>MHHHHHHGENLYFQGSEGEGVQLTAAQELMIQQLVAAQLQCNKRSFSDQPKVTPWPLGADPQSRDARQQRFAHFTELAIISVQE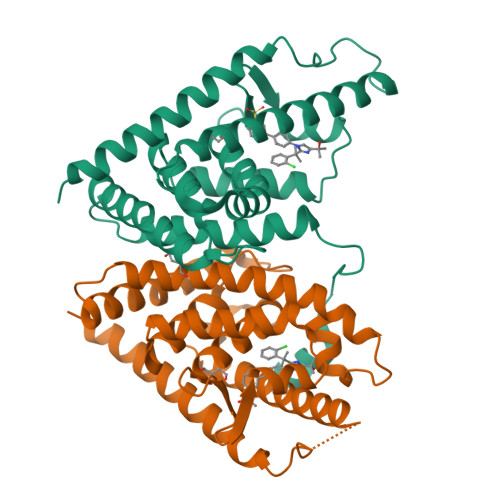IVDFAKQVPGFLQLGREDQIALLKASTIEIMLLETARRYNHETECITFLKDFTYSKDDFHRAGLQVEFINPIFEFSRAMRRLGLDDAEYALLIAINIFSADRPNVQEPGRVEALQQPYVEALLSYTRIKRPQDQLRFPRMLMKLVSLRTLSSVHSEQVFALRLQDKKLPPLLSEIWDVHE[2x]>MVLYFIGLGLYDER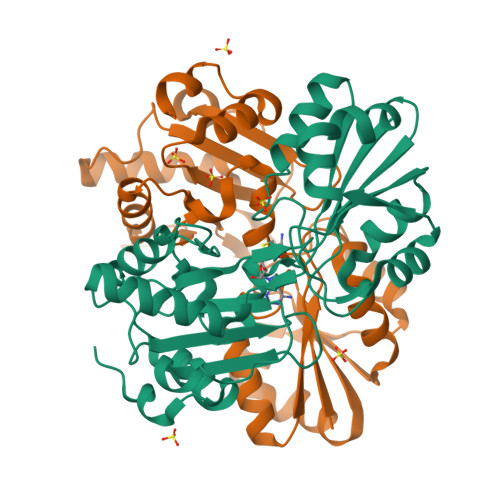DITVKGLEIAKKCDYVFAEFYTSLMAGTTLGRIQKLIGKEIRVLSREDVELNFENIVLPLAKENDVAFLTPGDPLVATTHAELRIRAKRAGVESYVIHAPSIYSAVGITGLHIYKFGKSATVAYPEGNWFPTSYYDVIKENAERGLHTLLFLDIKAEKRMYMTANEAMELLLKVEDMKKGGVFTDDTLVVVLARAGSLNPTIRAGYVKDLIREDFGDPPHILIVPGKLHIVEAEYLVEIAGAPREILRVNV[2x]> MGSSHHHHHHSSGTGSGENLYFQGHMSLSKKRKLESGDSGGAGAGGEGAEEENGGEQEAAPPRPRRTKSERDQLYYECYSDVSVHEEMIADQVRTEAYRLGILKNWAALRGKTVLDVGAGTGILSIFCAQAGARRVYAVEASAIWQQAREVVRLNGLEDRVHVLPGPVETVELPERVDAIVSEWMGYGLLHESM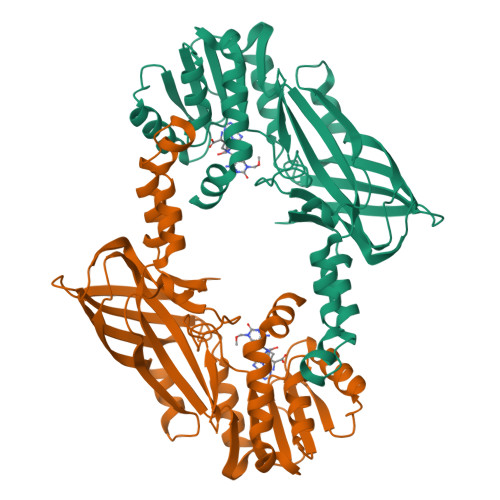LSSVLHARTKWLKEGGLLLPASAELFVAPISDQMLEWRLGFWSQVKQHYGVDMSCMESFATRCLMGHSEIVVQDLSGEDVLARPQRFAQLELARAGLEQELEAGVGGRFRCSCYGSAPLHGFAVWFQVTFPGGDSEKPLVLSTSPLHPATHWKQALLYLNEPVPVEQDTDISGEITLLPSPDNPRRLRILLRYKVGDHEEKTKDFAMED>[12x]MSDKLPTADSLRSMISGLGDPLRDKNASTFHWDRQLDDRQLLYAYRNSWVARKAVTIPALDAVRKWRDWQADQKDISRIEATEKRLGLQQKLLQCKTLARLWGGAAIVIGVKDQDMATPFEPETVNKDDLVYLTVMSRRELSPEELEQDPLDEFYARPKRYQVSNGRNLSFVHPSRIVHQVGETHPDPMLATGVNVGWGDSTLQALYDAMMNSDNTQANIASLVFEANVDVIGLPDFMENMSSEVYRQKLLDRFTLAAAG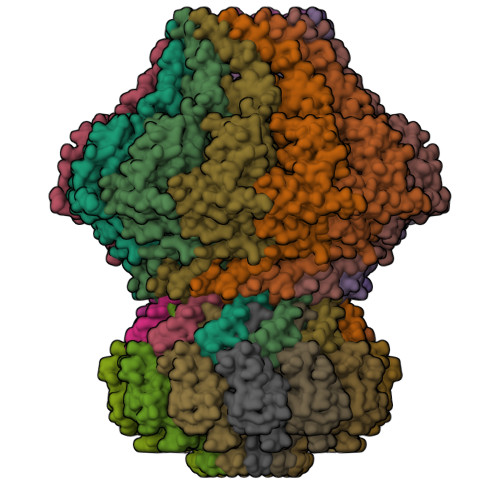KGINKTLMLDAEEVFTAHSRSFANLDKIMEQFILFVAGAADIPLTRFLGQSPAGMSSTGQHDMKNYHDRIQSIQTLDLQPSMYRLDEAIIRSSLGARPEELFYIWSPLEQMSEKERAEIGKLHAETVNVIAGTGLFMQEELREVFGNQLVETGLYPGLGDLLAQNGNELPEWDLEQRSAEASTKTAEAAALAAETASRQPARAVTDATPRPLYMRRDVVNGDEILRHYREQGVEGLYAAEELHVTIAYSKKPLDWMKLGEPWSAKLEVAPGGPRVHELFGDDSSVLVLCFAASELNWRAQQVIDAGGSSDHGEYQSHISLSLQGRPEQIETLRPYQGRIVLGPELFEQIEEGDWREKVKTD;>[12x]MNPIPAASDLKTRYPEFTGVSDAVVNAIIAEVNGMVDDGWEVSDQKPAVLALAAHMLSREGYPGRATNPNSFDPTNRPILSRKVGDVSTTFGRTDGGAAEGGANSYNYSSTVYGQTFLRLLRLNAPAVGLV> MSAKL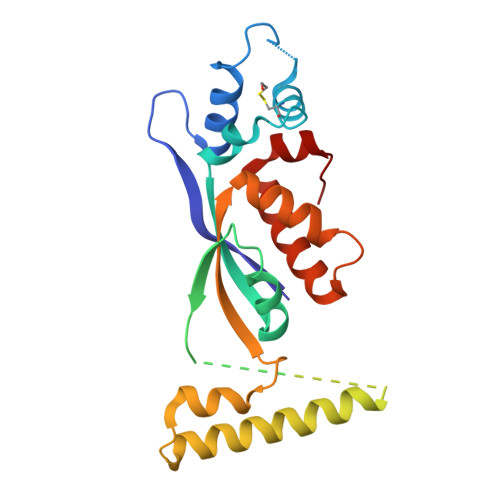ISVTKPVVEGVNTAEELIAYAARVSNPENQINNKTASGLLKYCIRHKHWSIFETAFMTLELKTSRGIAAQVLRHRSFHFQEFSQRYASVMETPPPHQARFQDHKNRQNSLDTVPEDDQTWWATEQEKLYAQSMELYNKALEKGIAKECARFILPLSTPTTIYMSGTIRDWIHYIELRTSNGTQREHIDLANACKEIFIKEFPSIAKALDWVH(2~{S})-1-[(3~{S})-3-[[(3~{S})-3,4-bis(oxidanyl)-4-oxidanylidene-butyl]amino]-4-oxidanyl-4-oxidanylidene-butyl]pyrrolidine-2-carboxylic 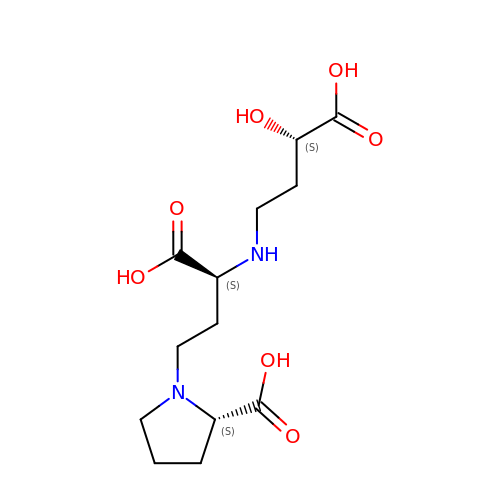acid | C13 H22 N2 O7 | OQMAZRGKYAMKSN-GUBZILKMSA-N CHOLIC ACID | C24 H40 O5 | 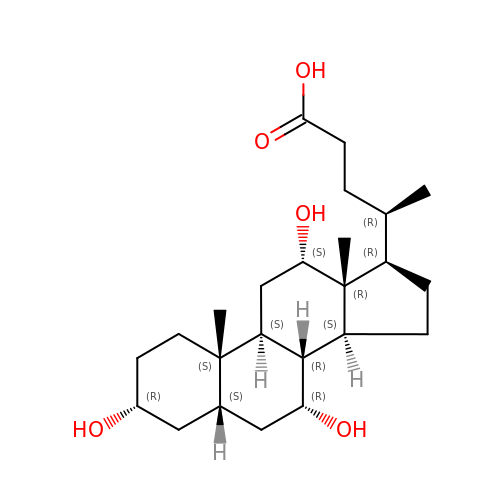BHQCQFFYRZLCQQ-OELDTZBJSA-N N-{[(1S)-1-carboxy-2-(4-hydroxy-3-iodophenyl)ethyl]carbamoyl}-L-glutamic acid | C15 H17 I N2 O8 | 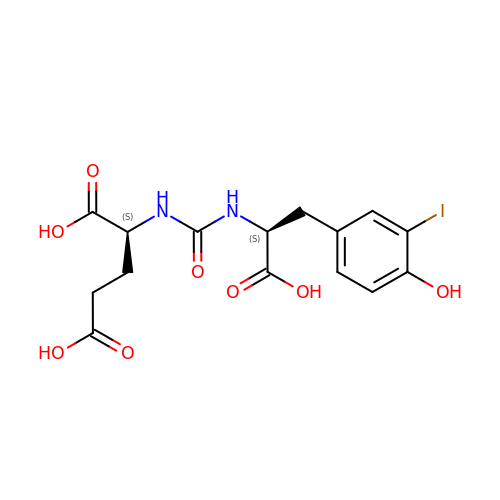GUNPTUQXZIVQBT-UWVGGRQHSA-N> GDNQDRTVANTQPSGPSNSTEIPALTAVETGHTSQVDPSDTIQTRHVVNFHSRSESTIENFMGRAACVFMDQYKINGEETSTDRFAVWTINIREMAQLRRKCEMFTYMRFDIEMTMVITSCQDQGTILDQDMPVLTHQIMYVPPGGPIPAKVDGYEWQTSTNPSVFWTEGNAPPRISIPFISVGNAY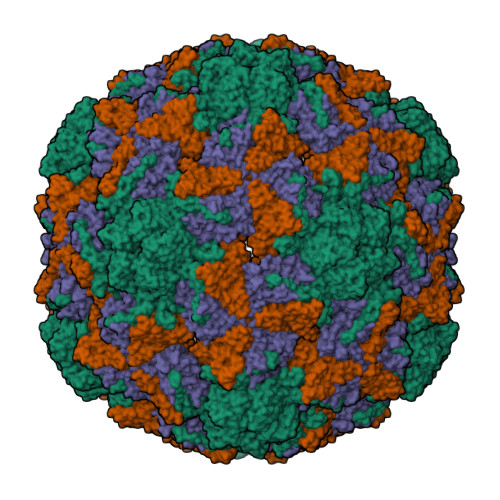SSFYDGWSHFTQDGTYGYTTLNAMGKLYIRHVNRSSPHQITSTIRVYFKPKHIKAWVPRPPRLCPYINKRDVNFVVTEITDSRTSITDTPHPEHSVLATH;> SPSAEECGYSDRVRSMTLGNSTITTQESANVVVGYGEWPSYLSDREATAEDQPTQPDVATCRFYTLESVQWEKTSPGWWWKFPEALKNMGLFGQNMHYHYLGRAGYTIHVQCNASKFHQGCLLVVCVPEAEMGCADTDTTFPATELTTEDTPHVFTSDSITGKKVQAAVCNAGMGVGVGNLTIFPHQWINLRTNNSATIVIPYINSVPMDNMFRHYNFTLMIIPFAPLNFTDGATAYVPITVTIAPMYAEYNGLRLASTQ;> GVPVLNTPGSNQFLTSDDYQSPSAMPQFDETPEMHIPGEVRNLMEIAEVDSVVPVNNVTGKTKSMDAYQIPVGTGNTDKTKPIFSFQMDPGYSSVLKRTLLGEMLNYYAHWSGSVKLTFLFCGSAMATGKLLISYSPPGASVPTSRKDAMLGTHIVWDIGLQSSCVLCVPWISQSHYRMVQQDPYTSAGYITCWYQTNIVVPPGAPTSCDVLCFASACNDFSVRLLRDTPFMAQPGKLQ>[3x]SKYVDRVIAEVEKKYADEPEFVQTVEEVLSSLGPVVDAHPEYEEVALLERMVIPERVIEFRVPWEDDNGKVHVNTGYRVQFNGAIGPYKGGLRFAPSVNLSIMKFLGFEQAFKDSLTTLPMGGAKGGSDFDPNGKSDREVMRFCQAFMTEL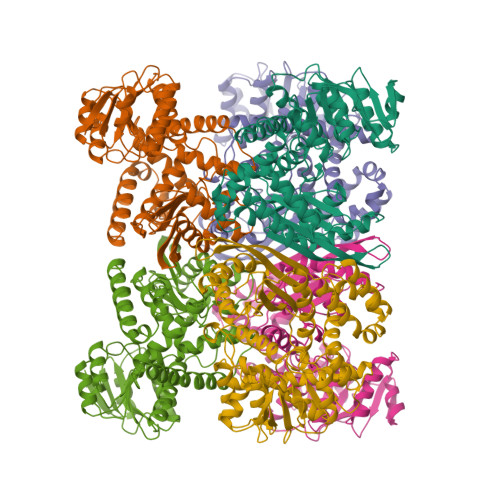YRHIGPDIDVPAGDLGVGAREIGYMYGQYRKIVGGFYNGVLTGKARSFGGSLVRPEATGYGSVYYVEAVMKHENDTLVGKTVALAGFGNVAWGAAKKLAELGAKAVTLSGPDGYIYDPEGITTEEKINYMLEMRASGRNKVQDYADKFGVQFFPGEKPWGQKVDIIMPCATQNDVDLEQAKKIVANNVKYYIEVANMPTTNEALRFLMQQPNMVVAPSKAVNAGGVLVSGFEMSQNSERLSWTAEEVDSKLHQVMTDIHDGSAAAAERYGLGYNLVAGANIVGFQKIADAMMAQGIAW>[4x]GIKCFAVRSLGWVEMTEEELAPGRSSVAVNNCIRQLSYHKNNLHDPMSGGWGEGKDLLLQLEDETLKLVEPQSQALLHAQPIISIRVWGVGRDSGR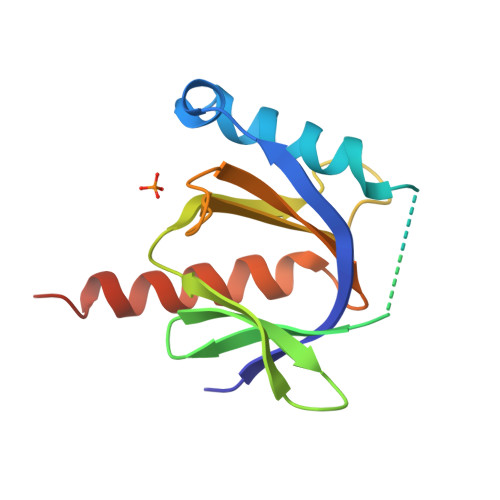ERDFAYVARDKLTQMLKCHVFRCEAPAKNIATSLHEICSKIMAELEHHHHHH[6-(phenylamino)-1-benzofuran-3-yl]acetic 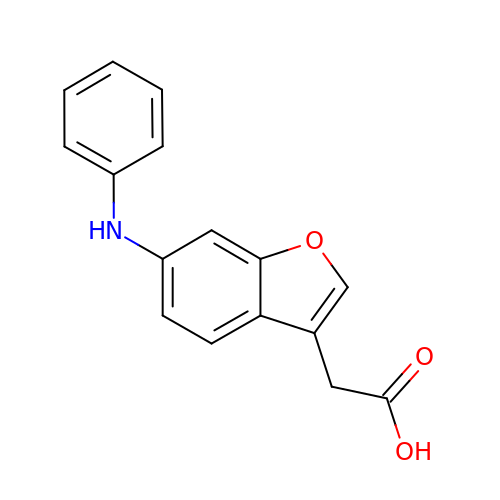acid | C16 H13 N O3 | OMQCVWMJZNPZAM-UHFFFAOYSA-N> ADPGTPGEAEGPACPAACVCSYDDDADELSVFCSSRNLTRLPDGVPGGTQALWLDGNNLSS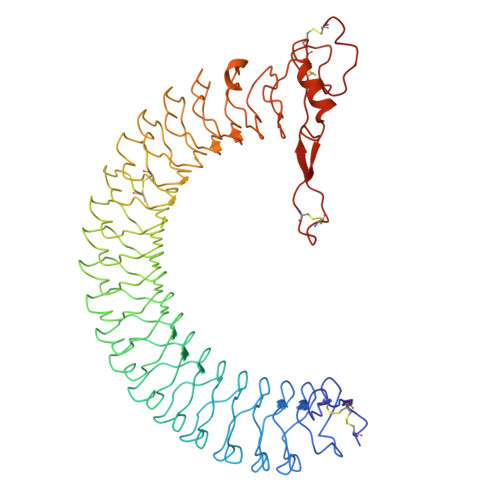VPPAAFQNLSSLGFLNLQGGQLGSLEPQALLGLENLCHLHLERNQLRSLALGTFAHTPALASLGLSNNRLSRLEDGLFEGLGSLWDLNLGWNSLAVLPDAAFRGLGSLRELVLAGNRLAYLQPALFSGLAELRELDLSRNALRAIKANVFVQLPRLQKLYLDRNLIAAVAPGAFLGLKALRWLDLSHNRVAGLLEDTFPGLLGLRVLRLSHNAIASLRPRTFKDLHFLEELQLGHNRIRQLAERSFEGLGQLEVLTLDHNQLQEVKAGAFLGLTNVAVMNLSGNCLRNLPEQVFRGLGKLHSLHLEGSCLGRIRPHTFTGLSGLRRLFLKDNGLVGIEEQSLWGLAELLELDLTSNQLTHLPHRLFQGLGKLEYLLLSRNRLAELPADALGPLQRAFWLDVSHNRLEALPNSLLAPLGRLRYLSLRNNSLRTFTPQPPGLERLWLEGNPWDCGCPLKALRDFALQNPSAVPRFVQAICEGDDCQPPAYTYNNITCASPPEVVGLDLRDLSEAHFAPC> MKATEQHYSIKEAMLFSQRIAQLSKALWKSIEKDWQRWIKPFDLNINEHHILWIAYHFKGASISEIAKFGVMHVSTAFNFSKKLEEKGLLSFSKKQDDKRNTYIELTEKGEEVLMKLMETYDPTKNAVFNGALPL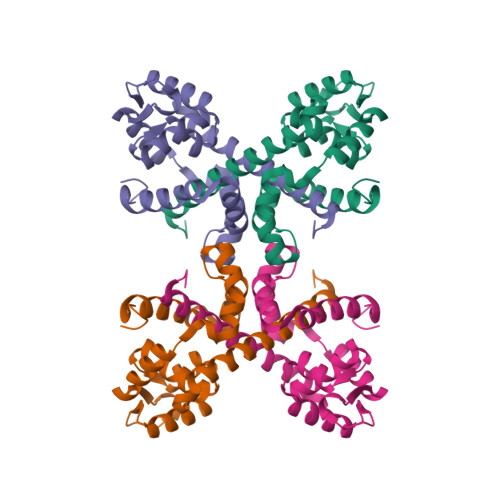RELYGKFPEILEMMCIVRNIYGDDFMEIFERAFENIKEDFIEQDGKLVKRKPKTEEHEKELASQANHHHHHH>MQAGPAMERHYYTYLIKEEFANHYFGRESVMFELFQDYHWTSLEKQQYEMTEKQIQYITQPIPILHMHQRLKMNLNKTDYRQLDYIYRIALPKAKGHATFMMKEHMIEIVASGDYEAETIFFEVLRKVSPCFLAMDFNSKRYGWLNPVKERNFV[2x];>GPAMENILDLWNQALAQIEKKLSKPSFETWMKSTKAHSLQGDTLTITAPNEFARDWLESRYLHLIADTIYELTGEELSIKFVIPQ[2x]

In prokaryotes, the DNA replication initiator protein is DnaA. SirA, a protein produced under Spo0A∼P regulation, has been identified as an inhibitor of DNA replication that plays a specific role in preventing replication re-initiation in cells committed to sporulation. Furthermore, the SirA binding determinants of DnaA have been mapped to its N-terminal domain, DnaADI. Here, we have solved the structure of SirA from B. subtilis in complex with DnaADI providing the first structure of a DnaA domain in an inhibitory complex.

The crystal structure of SirA–DnaADI was solved to 1.7 Å resolution using single anomalous dispersion (SAD) phasing techniques. SeMet-derivative crystals contain one complex per asymmetric unit (one molecule of SirA, one molecule of DnaADI) while the asymmetric unit of the native crystals contains two complexes. A vestigial N-terminal Gly-Pro-Ala sequence inherited from the DnaADI polyhistidine-tag can be seen in molecule D, and an additional N-terminal Ala is visible in molecule B. SirA–DnaADI is seen as a heterodimer, with molecules A (SirA) and B (DnaADI) forming one heterodimer and molecules C and D forming the other. SirA consists of a single globular domain comprising seven β-strands and five α-helices in the order β1-α1-α2-α3-α4-β2-β3-β4-β5-α5-β6-β7. DnaADI from B. subtilis consists of four alpha helices and three beta strands in the order α1-α2-β1-β2-α3-α4-β3 with a β-sheet topology of β1-β2-β3. The binding of SirA and DnaADI is mediated by helices α1, α2 and α3 of SirA and α2 and α3 of DnaADI. Seventeen residues on each chain contribute to the interface which constitutes 12% and 8% of the surface areas of DnaADI and SirA, respectively. In the complex, 1240 Å2 of otherwise accessible surface area is buried in the interface. In the SirA binding surface of DnaADI, Thr26, Trp27 and Phe49 contribute to the core of the interface with residues Pro22, Ser23, Glu25, Ser30, Pro46, Asn47, Glu48, Asp52, Ser56 and Trp53 prominent in the rim. On the corresponding DnaADI binding surface of SirA, Phe14, Tyr18, Gln48 and Ile52 contribute to the core and Glu13, His17, Val24, Leu28, Gln41, Met44, Lys47 and Tyr51 are prominent in the rim.> GHMQGQIIHHRNFQSQFDTTGNTLYNNAWVCSLNVIKSRDGNNYSALEDITSDNQAFNNILEGIDIIECENLLKEMNVQKIPESSLFTNIKEALQAEVFNSTVEDDFESFISYELQNHGPLMLIRPSLGSECLHAECIVGYDSEVKKVLIYDSMNTSPEWQSNIDVYDKLTLAFNDKYKNEDCSICGLYYDGVYEPK;> METREHL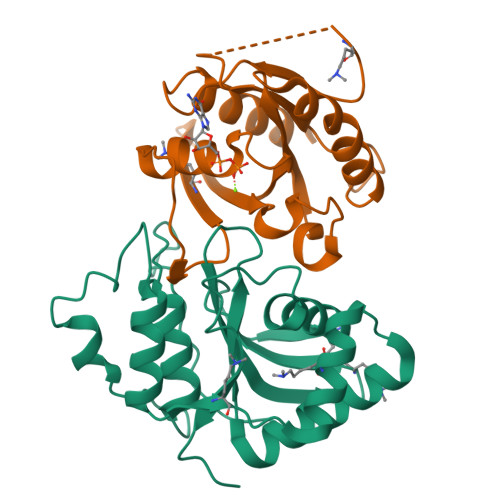FKVLVIGELGVGKTSIIKRYVHQLFSQHYRATIGVDFALKVLNWDSRTLVRLQLWDIAGQERFGNMTRVYYKEAVGAFVVFDISRSSTFEAVLKWKSDLDSKVHLPNGSPIPAVLLANKCDKNKDSSQSPSQVDQFDKEHGFAGWFETSAKDNINIEEAARFLVEKILVNHQSFPN> MRMFRITACVPSQTRIRTQRELQNTYFTKLVPYDNWFREQQRIMKMGGKIVKVELATGRPG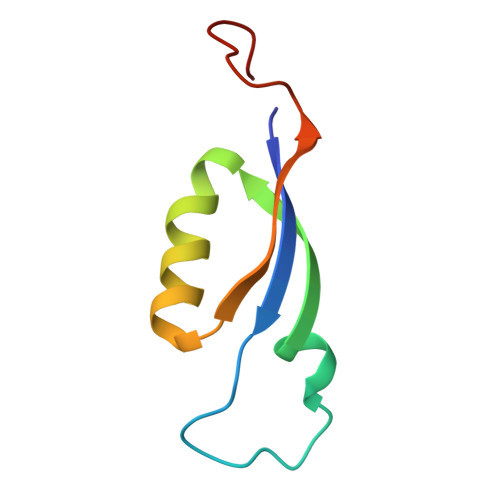TNAGLA> SQLLNEWSHNVDEL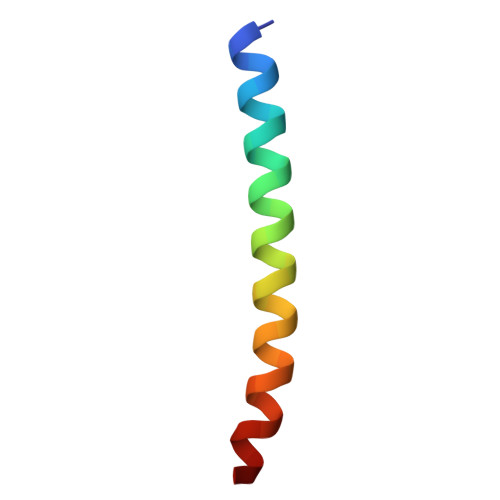LEHIETIGHLITKEEIMHGL> MAKKTSSKGRSSIPGPGYCMGIGPLISHGRFLWMGIGSACNYYNRVYGEFMRVWISGEETLIISKSS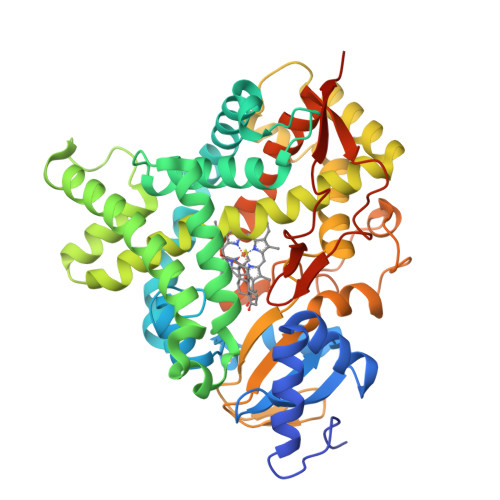SMFHIMKHNHYSSRFGSKLGLQCIGMHEKGIIFNNNPELWKTTRPFFMKALSGPGLVRMVTVCAESLKTHLDRLEEVTNESGYVDVLTLLRRVMLDTSNTLFLRIPLDESAIVVKIQGYFDAWQALLIKPDIFFKISWLYKKYEKSVKDLKDAIEVLIAEKRRRISTEEKLEECMDFATELILAEKRGDLTRENVNQCILEMLIAAPDTMSVSLFFMLFLIAKHPNVEEAIIKEIQTVIGERDIKIDDIQKLKVMENFIYESMRYQPVVDLVMRKALEDDVIDGYPVKKGTNIILNIGRMHRLEFFPKPNEFTLENFAKNVPYRYFQPFGFGPRGCAGKYIAMVMMKAILVTLLRRFHVKTLQGQCVESIQKIHDLSLHPDETKNMLEMIFTPRNSDRCLEHHHHH2-methyl-~{N}-[(1~{R})-1-[4-(methylsulfonylcarbamoyl)phenyl]ethyl]-5-phenyl-pyrazole-3-carboxamide 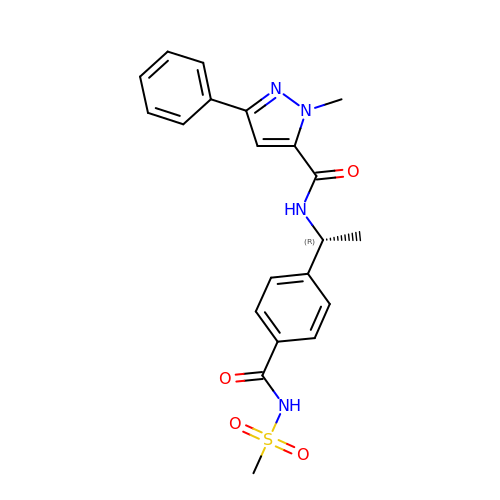| C21 H22 N4 O4 S | MRQUJSLINQBOAA-CQSZACIVSA-N> GSPGIPMVAAHAAHSQSSAEWIACLDKRPLERSSEDVDIIFTRLKGVKAFEKFHPNLLRQICLCGYYENLEKGITLFRQGDIGTNWYAVLAGSLDVKVSETSSHQDAVTICTLGIGTAFGESILDNTPRHATIVTRESSELLRIEQEDFKALWEKYRQYMAGLLAPPYGVMETGSNNDRIPDKENVPSEKILRAGKILRIAILSRAPHMIRD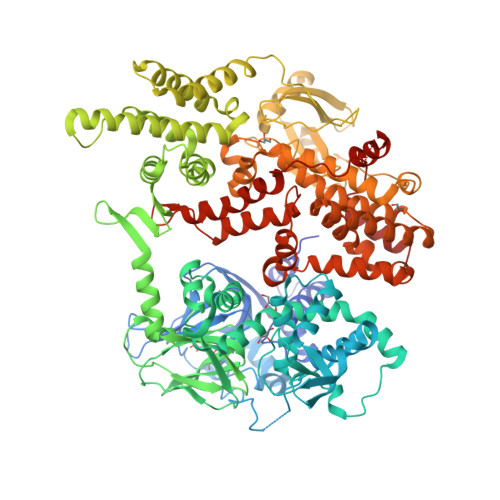RKYHLKTYRQCCVGTELVDWMIQQTSCVHSRTQAVGMWQVLLEDGVLNHVDQERHFQDKYLFYRFLDDEREDAPLPTEEEKKECDEELQDTMLLLSQMGPDAHMRMILRKPPGQRTVDDLEIIYDELLHIKALSHLSTTVKRELAGVLIFESHAKGGTVLFNQGEEGTSWYIILKGSVNVVIYGKGVVCTLHEGDDFGKLALVNDAPRAASIVLREDNCHFLRVDKEDGNRILRDVEANTVRLKEHDQDVLVLEKVPAGNRAANQGNSQPQQKYTVMSGTPEKILEHFLETIRLEPSLNEATDSVLNDFVMMHCVFMPNTQLCPALVAHYHAQPSQGTEQERMDYALNNKRRVIRLVLQWAAMYGDLLQEDDVAMAFLEEFYVSVSDDARMMAAFKEQLPELEKIVKQISEDAKAPQKKHKVLLQQFNTGDERAQKRQPIRGSDEVLFKVYCIDHTYTTIRVPVAASVKEVISAVADKLGSGEGLIIVKMNSGGEKVVLKSNDVSVFTTLTINGRLFACPREQFDSLTPLPEQEGPTTGTVGTFELMSSKDLAYQMTTYDWELFNCVHELELIYHTFGRHNFKKTTANLDLFLRRFNEIQFWVVTEVCLCSQLSKRVQLLKKFIKIAAHCKEYKNLNSFFAIVMGLSNVAVSRLALTWEKLPSKFKKFYAEFESLMDPSRNHRAYRLTAAKLEPPLIPFMPLLIKDMTFTHEGNKTFIDNLVNFEKMRMIANTARTVRYYRSQPFNPDAAQANKNHQDVRSYVRQLNVIDNQRTLSQMSHRLEPRRP>[2x]MEPSDQKVDTVPQYLKQSHERIFENNRA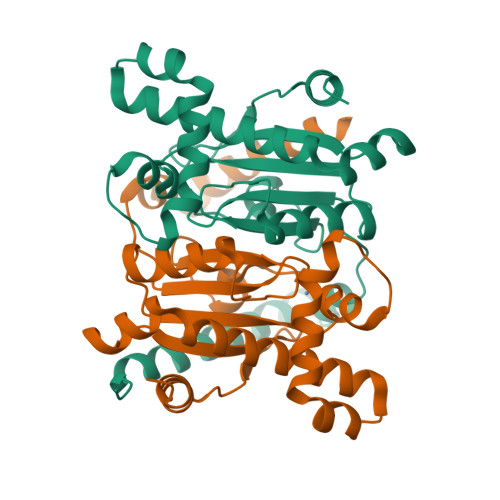WVATKMKDDPAFFEKLSAGQTPEYLYIGCSDSRVPANEIMGLEAGEVFVHRNIANLVPNTDLNVMSVINYAVRHLQVKHIVVCGHYHCGGVKAALTPSDLGLLNPWLRNVRDVYRLHEQELDGIQDATARARRLVELNVIESCRNVIKTAAVQQSFHERQFPVVHGWIFDVETGLLRDLEIDFEETLRDIKKIYNLAPGS> XHGLDDAQYLQQKAHNKRISEFRSSSNSGINVTVVLKYTNGVVQVYNWQGTEVIAGSLNRQLMKFPNYMNPDKHGRIEWPGEGVEHQHGLIRSNGGNGSYDIGAGDPYAMQFIVQGSVDWNATRLRFFGPDGSRWMPDDQGGASVRAGLLNAAEDIINSKMQPLYFCDRMAGKSYYVRFDDKYAPRFPTIGFEVYRYRVGATNEMGGESARTAVASLISFPTFSTAYVNEKVAVENFFQPRELVYQNSYGYTV

Cypoviruses, members of the family Reoviridae, subfamily Spinareovirus, possess a single capsid layer with turrets and are commonly embedded in crystalline occlusion bodies called polyhedra, which are formed in the cell cytoplasm and mainly composed of a single virus-encoded protein, polyhedrin. To ensure the delivery of virus particles to the target intestinal cells, allowing the transmission of packages of infectious virus between hosts by oral-faecal routes, polyhedra are disrupted only when they are exposed to the very alkaline pH environment found in insect midguts. The fold of all the polyhedrins is highly similar – a β-barrel core sitting on a base domain, surrounded by a common array of five helices (H1–H5). The strongest intermolecular interactions define a trimer composed of a cluster of three β-barrels sandwiched by helices top and bottom.

CPV5 has insertions at V3 and V2c which form two hairpins resembling a clamp. Despite a difference in unit cell of only ∼0.2 Å, native and SeMet crystals of CPV5 show a conformational change: in SeMet crystals pairs of loops 166–169 and 135–143 protrude to meet and coordinate a Ca2+ with Asp138 and Asp168, whilst in native CPV5 there is no evidence for the Ca2+, electron density is poor for 136–148, and the 135–143 loop shifts, possibly due to the proximity of methionine/SeMet residues at 136 and 170. There is no obvious significance to this change. The full length polyhedrin structures are generally well ordered, as expected for a crystal lattice which has extensive interactions and low solvent content (19–25%), however some types show regions of flexibility: 13 residues (136–148) of CPV5 and 6 residues (68–73) of CPV14 have high (>40 compared with an overall Wilson B-factor of 21.3) B-factors, whilst 13 residues (66–78) of CPV15 could not be modelled. In CPV5 V3 (179–187) and V2c (135–140) form clamp-like protrusions which fill the GTP and ATP pockets, whilst in the SeMet form a calcium ion links four polyhedrin molecules. CPV4 has limited numbers of molecular interactions in this area, while in CPV5 a few strong trimer-trimer interactions are present. The V5 regions of CPV5, 15, 17 and 19 differ, but all end in a similar place. In CPV1, 14, 15, 17, 18 and 20 solvent molecules can move between these two voids, whereas in CPV4, 5 and 19 they are blocked by tyrosine residues.> RICEVWACNLDEEMKKIRQVIRKYNYVAMDTEFPGVVARPIGEFRSNADYQYQLLRCNVDLLKIIQLGLTFMNEQG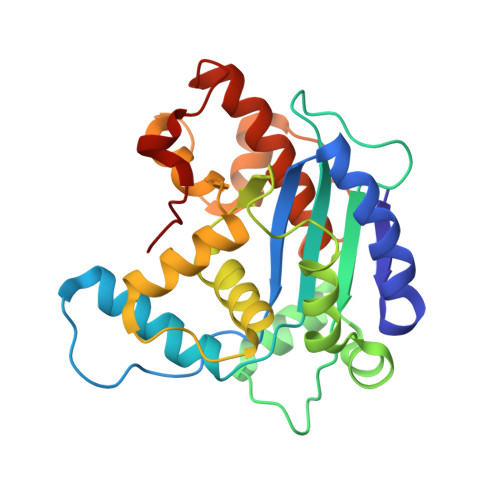EYPPGTSTWQFNFKFNLTEDMYAQDSIELLTTSGIQFKKHEEEGIETQYFAELLMTSGVVLCEGVKWLSFHSGYDFGYLIKILTNSNLPEEELDFFEILRLFFPVIYDVKYLMKSCKNLKGGLQEVAEQLELERIGPQHQAGSDSLLTGMAFFKMREMFFEDHIDDAKYCGHLYGL>[2x]IQNFYSLLGVSKTASSREIRQAFKKLALKLHPDKNPNNPNAHGDFLKINRAYEVLKDEDLRKKYDKYGEKGLEDNQGGQYESWSYYRYDFGIYDD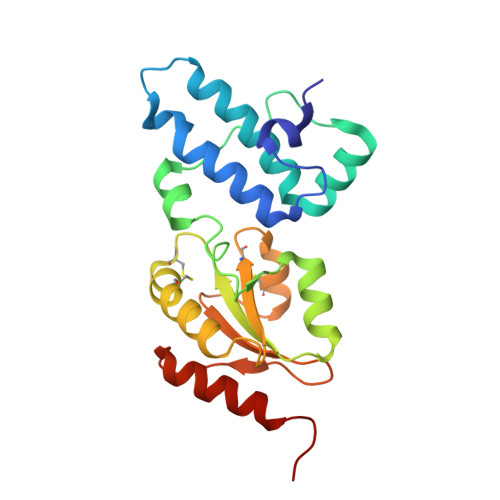DPEIITLERREFDAAVNSGELWFVNFYSPGCSHCHDLAPTWREFAKEVDGLLRIGAVNCGDDRMLCRMKGVNSYPSLFIFRSGMAAVKYNGDRSKESLVAFAMQHVRSTVTELST> MERRRLLHDGRWFTPCVLYGSARRGLKTLDVREYRPLAMPIEFRFYQRYANHPNRQSGIQFLTHYNTHQRFRVNKDYIDYMHWGKEQGQARLPHRHQRVAFDFNDQLHPTRIGTPEDGGNANHCYPEDGEDGSYAWFASQDPTFGHHPDLSSSFDPNYRVFSHPEHWNKMFTKRRPGEGDIDLSVLPSRSLLGPLMAHSDTKGIPYFKVDNRGHSNGRVPGVNAPFFGEFDQKMMQAMSRPLNANRTITGNDGRFSKTIMINEPQCNQALSAKTASELSKEIDKATNAVYSKLSVLEAAQSGLTDYFCGGLNFEIVGFELHMAAMLRERAAAILERSGAGGLPSASSATLSSSSTTRRCAMLLEKADEREVNKLLRDASRYEDRVDDALRQHASLIWRVYTAPRPLMTLTNGKCRGTGCGLSLFAKYCALKDSSEFIFDGPNVGITPYGGMT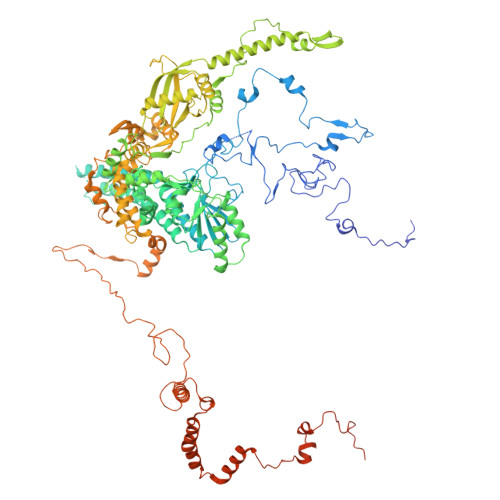RLLARPETSLKYPGLAEFVVLTGASLFAGDALRLGWTDLFTTIPDMTYHIKEWFDTTEHMHNDAVAWQLGHLLETCFKMKESHSSAMERAAITPTRARWVEDAFADQPSVNDIMRTLTEIEQLPFQSTHNTSDESHITPYTLGSVAAGVQRLGEHRLRYTLSPWDITPPEDSVVLKHTSEMFRAYVLERRGATDVVTHRDAERAAAWSQQRQREYDAYCSLKEAPHPRHVYARLEGCEGKIVSFEFVFEISCRRSGPQGTDEVLQTTTISRLKSRILDALGMPRDRNIDLGWYLPTLDTCPIHSDEELMQVLHTDPGIEDPKEKLRYPPIYFIVKRCTLYFSEWAYAVKHQLLLQSPFALRAAFGLLQEVRGDGAAENVMPLAETLGTEFKYFTRLMRRPDFYRVGVHTDKSVEKWEEIKEERRHNIHHTHRPTRPLPDFEEVFERDVEIDGHRFVLRPRWNPRTLQDVDDSDILRLRAPLTYDMDSTAALHVPTHCGKASRLAGMLQDAGGVQVLDGLGEVDDKGEPKVPPLQSNASVPTNVSFYEMARHPWEDRASSWRRDGFTEGSLEYFESQYRSAERAVYDEEGRGVRNYWPSRDAVEGIAQEEENDAQLLQERLFNTLETAGTSVEPWARNLRLNATTGKFGYKTEIATQEEKIYDDEYYRWFIQPGRHPNPSGLTLNGRKGQFEEGHSRDEELERMWRKVVADGNNDFAATTSGMPVYDEDAKNAEDSYAAGDDVDVVTTDANVPVDGDDSS>MAQGEKITVSNGVLNVPNNPIIPFIEGDGTGPDIWNAASKVLEAAVEKAYKGEKKITWKEVYAGEKAYNKTGEWLPAETLDVIREYFIAIKGPLTTPVGGGIRSLNVALRQELDLFVCLRPVRYFTGVPSPVKRPEDTDMVIFRENTEDIYAGIEYAKGSEEVQKLISFLQNELNVNKIRFPETSGIGIKPVSEEGTSRLVRAAIDYAIEHGRKSVTLVHKGNIMKFTEGAFKNWGYELAEKEYGDKVFTWAQYDRIAEEQGKDAANKAQSEAEAAGKIIIKDSIADIFLQQILTRPNEFDVVATMNLNGDYISDALAAQVGGIGIAPGANINYETGHAIFEATHGTAPKYAGLDKVNPSSVILSGVLLLEHLGWNEAADLVIKSMEKTIASKVVTYDFARLMDGAT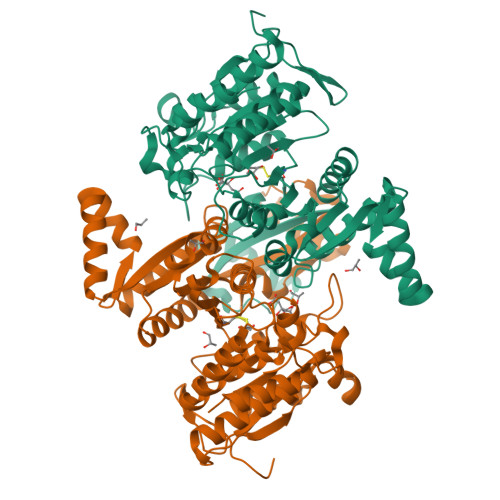EVKCSEFGEELIKNMD[2x]> MEHVAFGSEDIENTLAKMDDGQLDGLAFGAIQLDGDGNILQYNAAEGDITGRDPKQVIGKNFFKDVAPCTDSPEFYGKFKEG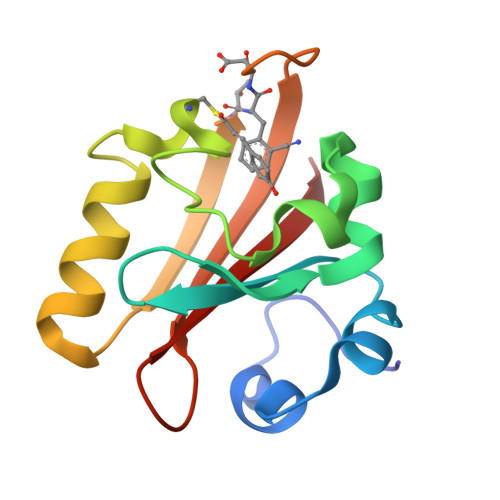VASGNLNTMFEYTXDYQHTPTKVKVHMKKALSGDSYWVFVKRV>[2x]GSLFDPSCTGVFDR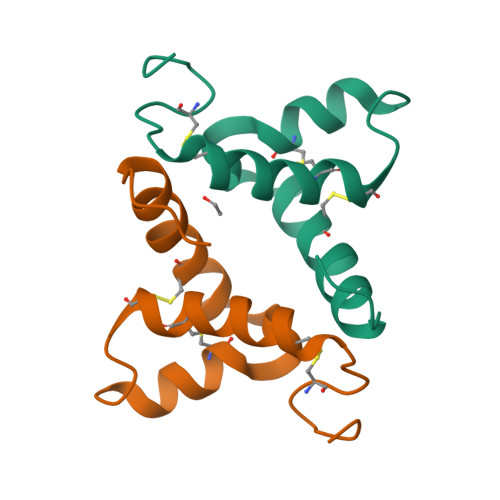QLLRRLGRVCDDCFNVFREPNVATECRSNCYNNPVFRQCMAYVVPAHLHNEHREAVQMVG N-[(1S,2R)-2-azanylcyclohexyl]-5-[2-[(3,5-dimethylphenyl)amino]pyrimidin-4-yl]-2-methyl-pyrazole-3-carboxamide | C23 H29 N7 O | 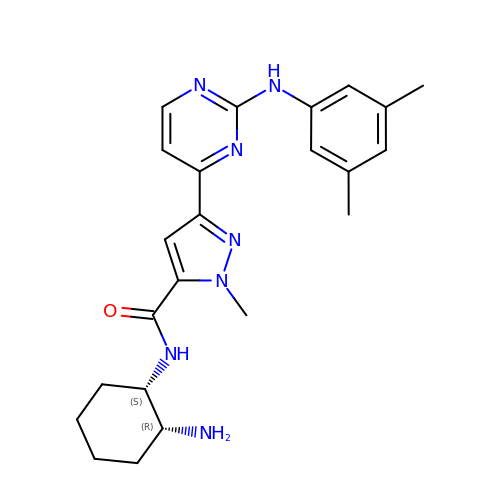DEYILQIXALFSOO-MSOLQXFVSA-N>MAHHHHHHMRIVINGFGRIGRLVLRQILKRNSPIEVVAINDLVAGDLLTYLFKYDSTHGSFAPQATFSDGCLVMGERKIRFLAEKDVQKLPWKDLDVDVVVESTGLFVNRDDAAKHLDSGAKRVLITAPAKGDVPTFVMGVN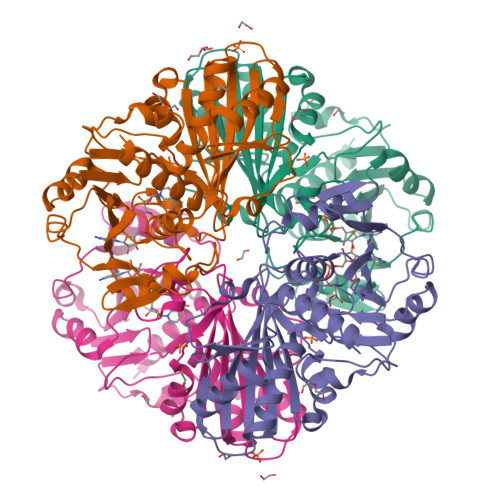HQQFDPADVIISNASCTTNCLAPLAKVLLDNFGIEEGLMTTVHAATATQSVVDGPSRKDWRGGRGAFQNIIPASTGAAKAVGLCLPELKGKLTGMAFRVPVADVSVVDLTVKLSSATTYEAICEAVKHAANTSMKNIMYYTEEAVVSSDFIGCEYSSIFDAQAGVALNDRFFKLVAWYDNEIGYATRIVDLLEYVQENSK[4x]>[24x]MLYRGLRMAARAAPKFAVLNTHAALRQLPLQFQHVRT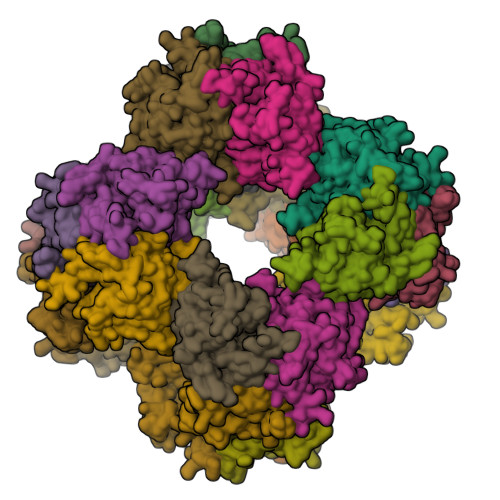YADKIIKVPQMAESITEGTLKQWNKAVGDYVEADEEIATIETDKIDVAVNAPEAGVIKEFFVNEEDTVLVGQDLVRLEVGGEKPAEAAKEQPKAAAPEPKVEEKKVPEAPAPEPSKTAAPAPAPPKQEAPASPKPASKPAETPAVTLGNREERRVKMNRMRLRIAERLKQSQNTAASLTTFNEVDMSALIEFRNKYKDEVLKKTGVKLGFMSAFSRAVVLAIRDLPVVNASIEGPNGGDTIVYRDYVDISVAVATEKGLVTPVVRNAETMDLITIEKTIAELGKKARDGKLTIEDMAGGTFTISNGGVFGSLMGTPIINLPQSAVLGLHAIKERPVAVNGKVEIRPMMYLALTYDHRLLDGREAVQFLVKVKEYIEDPRKMLL> SFESKK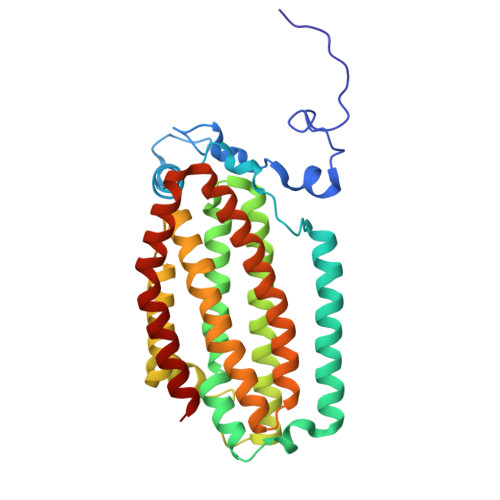PMRTWSHLAEMRKKPSEYDIVSRKLHYSTNNPDSPWELSPDSPMNLWYKQYRNASPLKHDNWDAFTDPDQLVYRTYNLMQDGQESYVQSLFDQFNEREHDQMVREGWEHTMARCYSPLRYLFHCLQMSSAYVQQMAPASTISNCCILQTADSLRWLTHTAYRTHELSLTYPDAGLGEHERELWEKEPGWQGLRELMEKQLTAFDWGEAFVSLNLVVKPMIVESIFKPLQQQAWENNDTLLPLLIDSQLKDAERHSRWSKALVKHALENPDNHAVIEGWIEKWRPLADRAAEAYLSMLSS>GHMALSLANYLAADSAAEALRRDVRAGLTATQKSLPPKWFYDAVGSDLFDQITRLPEYYPTRTEAQILRTRSAEIISAAGADTLVELGSGTSEKTRMLLDAMRDAELLRRFIPFDVDAGVLRSAGAAIGAEYPGIEIDAVCGDFEEHLGKIPHVGRRLVVFLGSTIGNLTPAPRAEFLSTLADT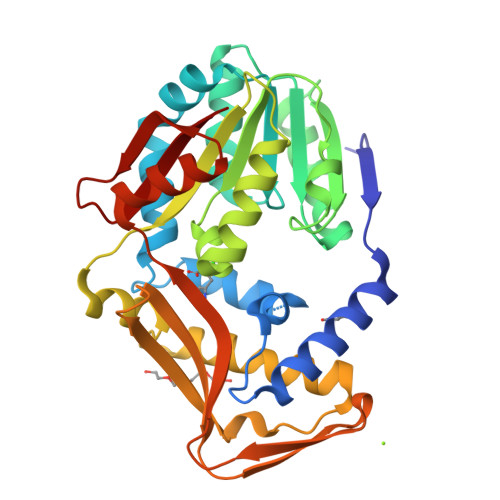LQPGDSLLLGTDLVKDTGRLVRAYDDAAGVTAAFNRNVLAVVNRELSADFDLDAFEHVAKWNSDEERIEMWLRARTAQHVRVAALDLEVDFAAGEEMLTEVSCKFRPENVVAELAEAGLRQTHWWTDPAGDFGLSLAVR[2x]>MADKIKDAKIIFVVGGPGSGKGTQCEKIVAKYGYTHLSSGDLLRAEVSSGSERGKQLQAIMQKGELVPLDTVLDMIKDAMIAKADVSKGYLIDGYPREVKQGEEFEKKIGKPCLLLYIDAKGETMVKRLMKRGETSGRADDNEETIKKRLDLYY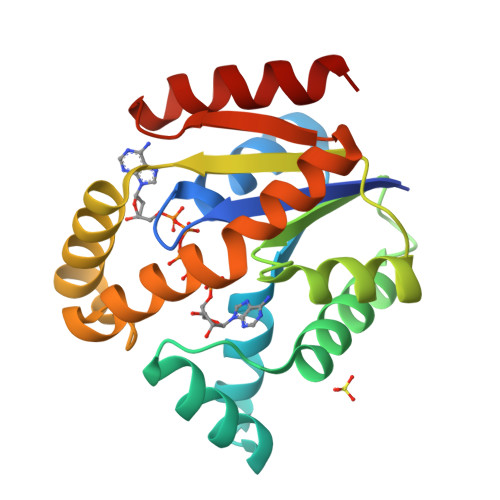KATEPVIAFYEGRGIVRKIDSELPVDEVFKQVSTAIDAL[2x]>GSMPKPINVRVTTMDAELEFAIQPNTTGKQLFDQVVKTVGLREVWFFGLQYVDSKGYSTWLKLNKKVTQQDVKKENPLQFKFRAKFFPEDVSEELIQEITQRLFFLQVKEAILNDEIYCPPETAVLLASYAVQAKYGDYNKEIHKPGYLANDRLLPQRVLEQHKLTKEQWEERIQNWHEEHRGMLREDSMMEYLKIAQDLEMYGVNYFEIKNKKGTELWLGVDALGLNIYEHDDKLTPKIGFPWSEIRNISFNDKKFVIKPIDKKAPDFVFYAPRLRINKRILALCMGNHELYMRRRKPDTIEVQQMKAQAR[4x];>KERAHQKRSS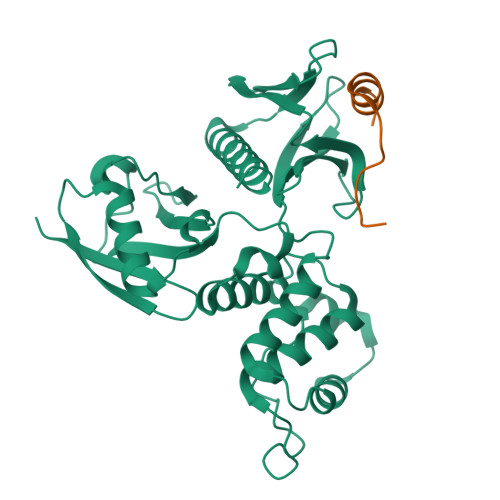KRAPQMDWSKKNELFSNL[4x]>[4x]SMKLSEQLKHCNGILKELLSKKHAAYAWPFYKPVDASALGL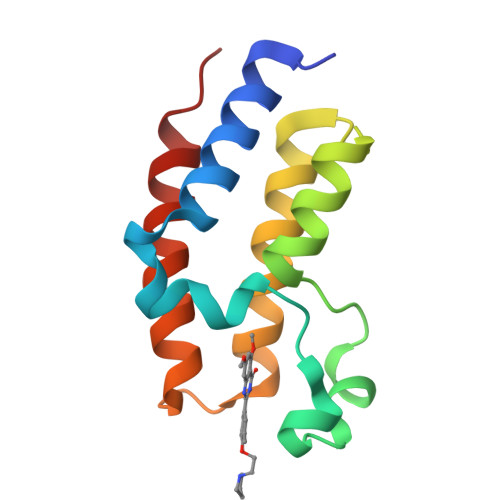HDYHDIIKHPMDLSTVKRKMENRDYRDAQEFAADVRLMFSNCYKYNPPDHDVVAMARKLQDVFEFRYAKMPD Poxviruses are large DNA viruses which replicate exclusively in the cytosol, and encode poxvirus immune nucleases (poxins) to degrade 2′3′-cGAMP and prevent STING activation (Eaglesham et al., 2019). While baculovirus and lepidopteran poxin homologs share <25% identity with VACV poxin, they are functional nucleases and retain 2′3′-cGAMP-specific cleavage activity. New poxin structures include the alphabaculovirus Autographa californica nucleopolyhedrovirus (AcNPV) poxin from Group 2, lepidopteran host poxins from the moth Trichoplusia ni and the monarch butterfly Danaus plexippus in Group 3, and the betabaculovirus Pieris rapae granulovirus (PrGV) poxin from Group 4. In spite of dramatic sequence divergence, poxin structures from each group reveal a shared core fold and head-to-tail dimeric architecture confirming poxins as a single enzyme family.

Group two primarily contains poxins encoded in alphabaculovirus genomes. The new poxin structures trap a post-reaction state following 2′3′-cGAMP cleavage and allow direct comparison with the catalytic mechanism of VACV poxin. Strikingly, despite sharing <21% identity, each poxin structure contorts 2′3′-cGAMP in an identical strained conformation. Consistent with specificity for 2′3′-cGAMP and a shared mechanism of catalysis, the active-site charge landscape is conserved across all poxin proteins, with hydrophobic pockets for the bases, and multiple basic residues stabilizing the negatively charged phosphates of the 2′3′-cGAMP ligand. Unlike the catalytic triad of histidine, tyrosine, and lysine residues essential for VACV and AcNPV poxin cleavage activity, the active sites of T. ni poxin and PrGV poxin are divergent. Interestingly, mammalian and insect viral poxins from VACV and AcNPV exhibit similar kinetics, with a KM of 0.83 µM and 2.43 µM respectively, while the T. ni host poxin protein has a KM two orders of magnitude higher at 342.1 µM. Consistent with our enzyme kinetics results, inactive VACV and AcNPV poxin exhibited a KD of 0.58 µM and 0.81 µM respectively, within a similar range as the respective KM values of wild-type enzymes. Comparison of lepidopteran poxins with viral poxins from AcNPV and VACV reveals greater degeneration in the protease domain and protease active-site pocket in viral enzymes that results in loss of C-terminal coordination.

>[16x]SMELYNIKYAIDPTNKIVIEQVDNVDAFVHILEPGQEVFDETLSQYHQFPGVVSSIIFPQLVLNTIISVLSEDGSLLTLKLENTCFNFHVCNKRFVFGNLPAAVVNNETKQKLRIGAPIFAGKKLVSVVTAFHRVGENEWLLPVTGIREASQLSGHMKVLNGVRVEKWRPNMSVYGTVQLPYDKIKQHALEQENKTPNALESCVLFYKDSEIRITYNKGDYEIMHLRMPGPLIQPNTIYYS DHFR is an enzyme vital for cellular replication, mainly due to its important role in the one-carbon metabolism pathway. DHFR reduces dihydrofolate (DHF) to tetrahydrofolate (THF). Nicotinamide adenine dinucleotide phosphate (NADPH) is required for this catalytic reaction. The mutation F98Y in Staphylococcus aureus dihydrofolate reductase (SaDHFR) confers resistance to the clinically important antifolate trimethoprim (TMP).

At that time, the NADPH in R-27 complex was thought to be in its α configuration (α-NADPH). Further refinement of the SaDHFR:R-27 structure was needed to assess the fit of t-NADPH into the NADPH binding site. Upon refinement of these two structures in phenix, we observed that the t-NADPH cofactor better satisfied both the local electron density map and difference density that arose in the α-NADPH structure. Additionally, we observe a decrease in the average cofactor B-factors (from 39.98 with α-NADPH to 33.55 with t-NADPH) and the B-factors of the oxygen atom involved in cyclization (from 39.22 with α-NADPH to 34.15 with t-NADPH). Furthermore, there is an overall decrease in Rfree for the structure with the remediation of the NADPH cofactor, with a decrease from 0.2543 with α-NADPH to 0.2529 with t-NADPH, a meaningful decrease given the minor structural differences between cofactor structures. Computing difference density based on the original assignment of α-NADPH revealed an unsatisfied region of density at the site of ring-closure, which is satisfied by reassignment of t-NADPH. Thus, we created two new, improved structure models with significant implications in terms of biological physical chemistry (discussed herein). Both new structures were deposited in the PDB.

> TLSILVAHDLQRVIGFENQLPWHLPNDLKHVKKLSTGHTLVMGRKTFESIGKPLPNRRNVVLTSDTSFNVEGVDVIHSIEDIYQLPGHVFIFGGQTLFEEMIDKVDDMYITVIEGKFRGDTFFPPYTFEDWEVASSVEGKLDEKNTIPHTFLHLIRK> AQPDIKFASKEYGVTIGESRIIYPLDAAGVMVSVKNTQDYPVLIQSRIYDENKEKESEDPFVVTPPLFRLDAKQQNSLRIAQAGGVFPRDKESLKWLCVKGIPPKDEDIWVDDATNKQKFNPDKDVGVFVQFAINNCIKLLVRPNELKGTPIQFAENLSWKVDGGKLIAENPSPFYMNIGELTFGGKSIPSHYIPPKSTWAFDLPKGLAGARNVSWRIINDQGGLD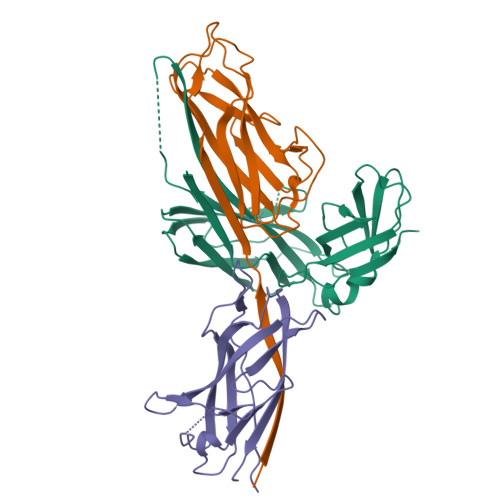RLYSKNVTL;> ADLTASTTRTATLVEPARITLTYKEGAPITIMDNGNIDTELLVGTLTLGGYKTGTTSTSVNFTDAAGDPMYLTFTSQDGNNHQFTTKVIGKDSRDFDISPKVNGENLVGDDVVLATGSQDFFVRSIGSKGGKLAAGKYTDAVTVTVSNQ;> ADLTSHHHHHHVEPARITLTYKEGAPITIMDNGNIDTELLVGTLTLGGYKTGTTSTSVNFTDAAGDPMYLTFTSQDGNNHQFTTKVIGKDSRDFDISPKVNGENLVGDDVVLATGSQDFFVRSIGSKGGKLAAGKYTDAVTVTVSNQ>PVTLEPMPPGEGAQEGEPPTVEARYKSFSIKMLKDMKEGVKQYGPNSPYMRTLLDSIAHGHRLIPYDWEILAKSSLSPSQFLQFKTWWIDGVQEQVRRNRAANPPVNIDADQLLGIGQNWSTISQQALMQNEAIEQVRAICLRAWEKIQDPGSACPSFNTVRQGSKEPYPDFVARLQDVAQKSIADEKARKVIVELMAYENANPEC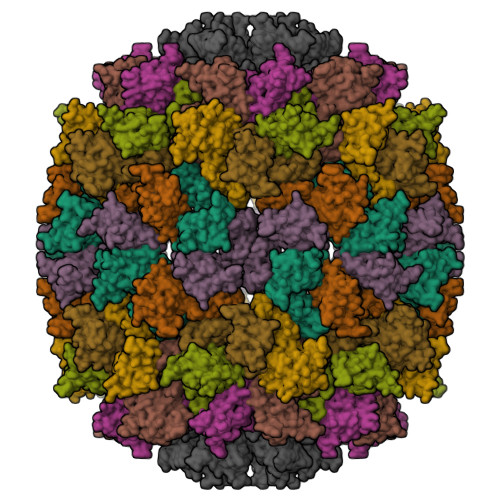QSAIKPLKGKVPAGSDVISEYVKACDGIGGAMHKAMLMAQLE[9x]>NFDAERDALNIETAIKTKGVDEVTIVNILTNRSNAQRQDIAFAYQRRTKKELASALKSALSGHLETVILGLLKTPAQYDASELKASMKGLGTDEDSLIEIICSRTNQELQEINRVYKEMYKTDLEKDIISDTSGDFRKLMVALAKGRRAEDGSVIDYELIDQDARDLYDAGVKRKGTDVPKWISIMTERSVPHLQKVFDRYKSYSPYDMLESIRKEVKGDLENAFLNLVQCIQNKPLYFADRLYD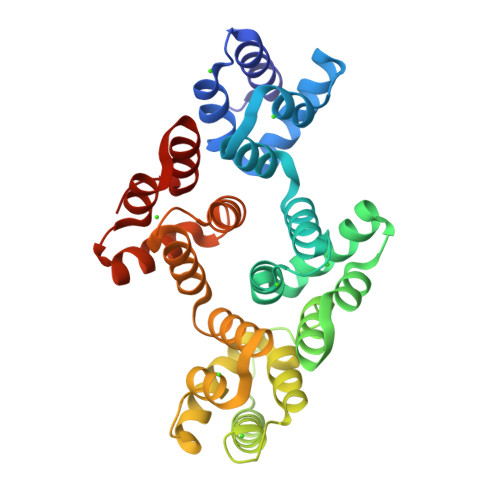SMKGKGTRDKVLIRIMVSRSEVDMLKIRSEFKRKYGKSLYYYIQQDTKGDYQKALLYLCGGDD[2x]>MGVHTFEEESTSPVPPAKLFKATVVDGDELTPKLIPAIQSIEIVEGNGGPGTVKKVTAVEDGKTSYVLHKIDAIDEATYTYDYTISGGTGFQEILEKVSFKTKLEAADGGSKIKVSVTFHTKGDAPLPDEVHQDVKQKSQGIFKA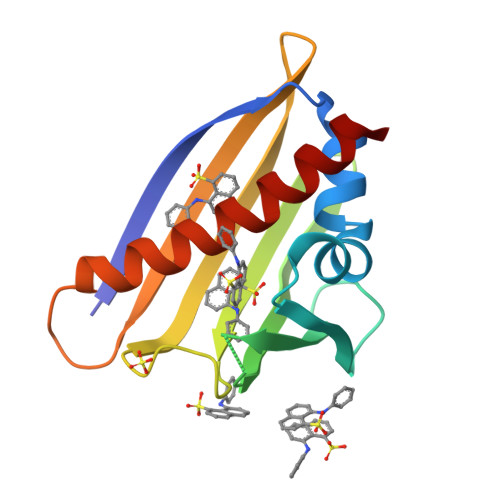IEGYVLSN[2x]> GSSMGSDEQRRELEEKIKLKLEELKTKSEEERKEIKLRVIAYVLVQLEDLQKNLSDEQRRELEEKIKAKLEELKTKSEEERKEIKLRVIAYVLVQLEDLQKNLSDEQRRELEEKIKWKLEELKTKSEEERKEIKLRVIA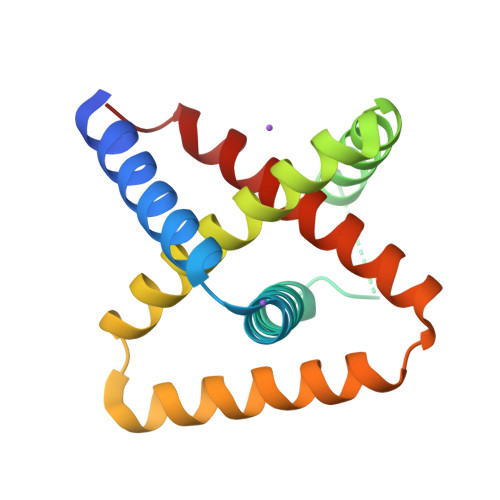YVLVQLEDLQKNLS>MGSTSTPDSSTNRLQDKVAIITGGAGGIGETTAKLFVRYGAKVVIADIADDHGQKVCNNIGSPDVISFVHCDVTKDEDVRNLVDTTIAKHGKLDIMFGNVGVLSTTPYSILEA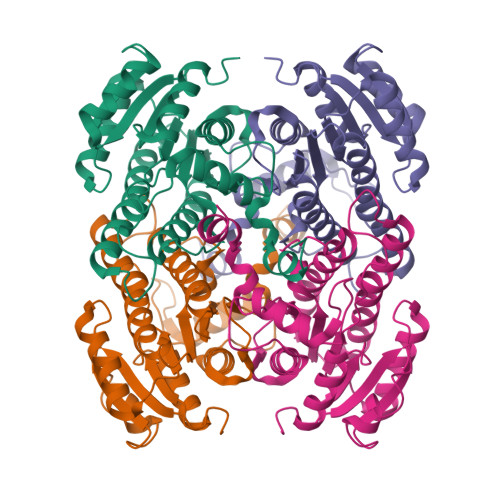GNEDFKRVMDINVYGAFLVAKHAARVMIPAKKGSIVFTASISSFTAGEGVSHVYTATKHAVLGLTTSLCTELGEYGIRVNCVSPYIVASPLLTDVFGVDSSRVEELAHQAANLKGTLLRAEDVADAVAYLAGDESKYVSGLNLVIDGGYTRTNPAFPTALKHGLA[2x]>GCCGGACGG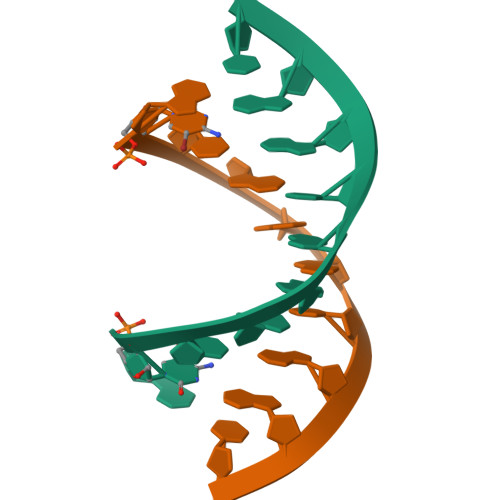C[2x]> MDNSVETIELKRGSNSVYVQYDDIMFFESSTKSHRLIAHLDNRQIEFYGNLKELSQLDDRFFRCHNSF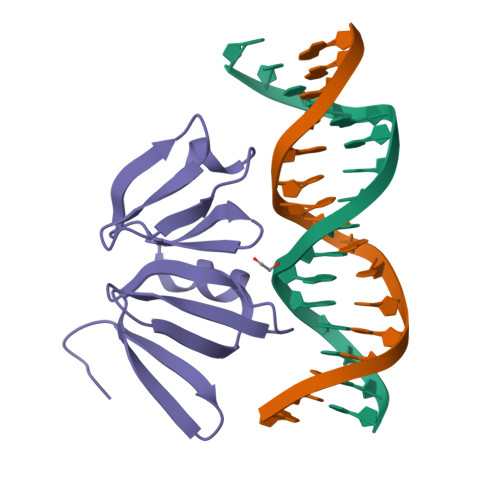VVNRHNIESIDSKERIVYFKNKEHCYASVRNVKKI>MGSDKIHHHHHHMKVFTEKIPNIPWEERPEGYTGPVWRYSKNPIIGRNPVPKGARVFNSAVVPYNGEFVGVFRIDHKNTRPFLHFGRSKDGINWEIEPEEIQWVDVNGEPFQPSY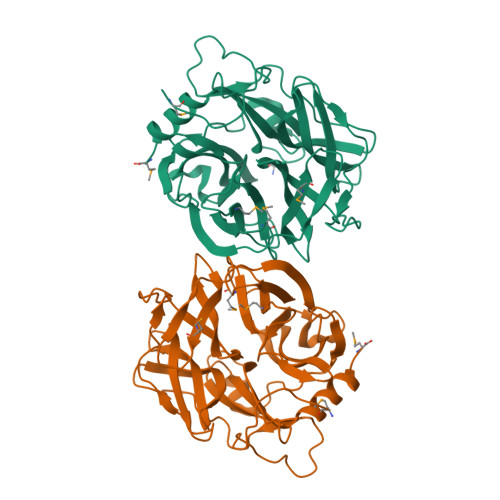AYDPRVVKIEDTYYITFCTDDHGPTIGVGMTKDFKTFVRLPNAYVPFNRNGVLFPRKINGKYVMLNRPSDNGHTPFGDIFLSESPDMIHWGNHRFVLGRSSYNWWENLKIGAGPYPIETSEGWLLIYHGVTLTCNGYVYSFGAALLDLDDPSKVLYRSRYYLLTPEEEYETVGFVPNVVFPCAALCDADTGRVAIYYGAADTHVALAFGYIDEIVDFVKRNSM[6x]> NQSVVVDFLLPTGVYLNFPVSRNANLSTIKQLLWHRAQYEPLFHMLSGPEAYVFTCINQTAEQQELEDEQRRLCDVQPFLPVLRLVAREGDRVKKLINSQISLLIGKGLHEFDSLCDPEVNDFRAKMCQFCEEAAARRQQLGWEAWLQYSFPLQLEPSAQTWGPGTLRLPNRALLVNVKFEGSEESFTFQVSTKDVPLALMACALRKKATVFRQPLVEQPEDYTLQVNGRHEYLYGSYPLCQFQYICSCLHSGLTPHLTMVHSSSILAMRDEQSNPAPQVQKPRAKPPPIPAKKPSSVSLWSLEQPFRIELIQGSKVNADERMKLVVQAGLFHGNEMLCKTVSSSEVSVCSEPVWKQRLEFDINICDLPRMARLCFALYAVIEKAKKARSTKKKSKKADCPIAWANLMLFDYKDQLKTGERCLYMWPSVPDEKGELLNPTGTVRSNPNTDSAAALLICLPEVAPHPVYYPALEKILELGRHSECVHVTEEEQLQLREILERRGSGELYEHEKDLVWKLRHEVQEHFPEALARLLLVTKWNKHEDVAQMLYLLCSWPELPVLSALELLDFSFPDCHVGSFAIKSLRKLTDDELFQYLLQLVQVLKYESYLDCELTKFLLDRALANRKIGHFLFWHLRSEMHVPSVALRFGLILEAYCRGSTHHMKVLMKQGEALSKLKALNDFVKLSSQKTPKPQTKELMHLCMRQEAYLEALSHLQSPLDPSTLLAEVCVEQCTFMDSKMKPLWIMY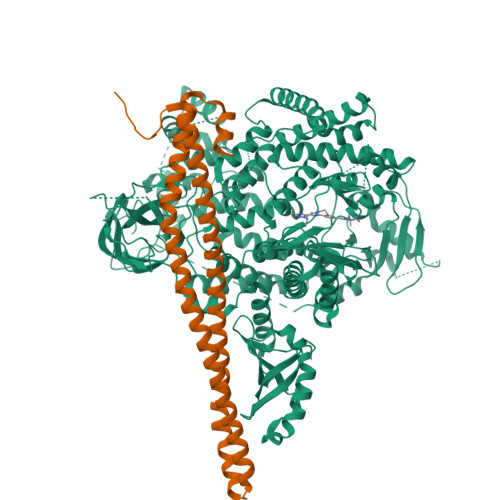SNEEAGSGGSVGIIFKNGDDLRQDMLTLQMIQLMDVLWKQEGLDLRMTPYGCLPTGDRTGLIEVVLRSDTIANIQLNKSNMAATAAFNKDALLNWLKSKNPGEALDRAIEEFTLSCAGYCVATYVLGIGDRHSDNIMIRESGQLFHIDFGHFLGNFKTKFGINRERVPFILTYDFVHVIQQGKTNNSEKFERFRGYCERAYTILRRHGLLFLHLFALMRAAGLPELSCSKDIQYLKDSLALGKTEEEALKHFRVKFNEALRESWKTKV;> YQQDQVVKEDNIEAVGKKLHEYNTQFQEKSREYDRLYEDYTRTSQEIQMKRTAIEAFNETIKIFEEQCQTQERYSKEYIEKFKREGNETEIQRIMHNYEKLKSRISEIVDSRRRLEEDLKKQAAEYREIDKRMNSIKPDLIQLRKTRDQYLMWLTQKGVRQKKLNEWLG> EIASEYLGGPGGDAFDDKAVAQNGDITRIEMQCTDVATYIKLRYGKVDSRQWGWGNE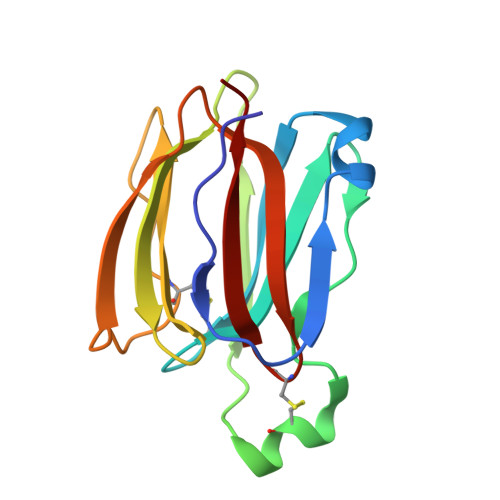NCIQWSKKGEKVVHELSSGEYITSAIVTYGKYVQSITFKTNKRTLPRCGTSATEKSVTVLIPGGLKYISGRWGCRIDGLRFHAKC>[2x]MALPKPPGTPVVTESTATSITLTWDSGNPEPVSYYIIQHKPKNSEEPYKEIDGIATTRYSVAGLSPYSDYEFRVVAVNNIGRGPASEPVLTQTSEQAPSSAPRDVQARMLSSTTILVQW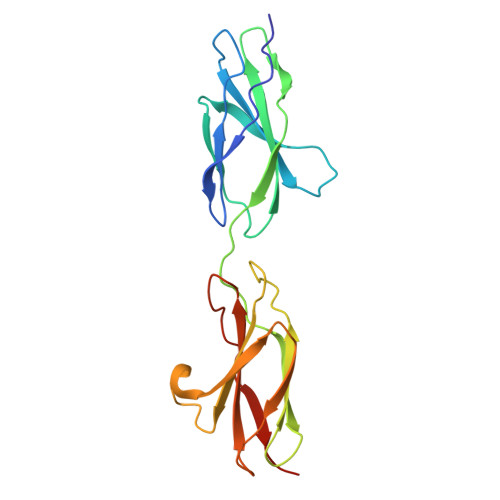KEPEEPNGQIQGYRVYYTMDPTQHVNNWMKHNVADSQITTIGNLVPQKTYSVKVLAFTSIGDGPLSSDIQVITLEHHHHHH> GKPRPYSPRPTSH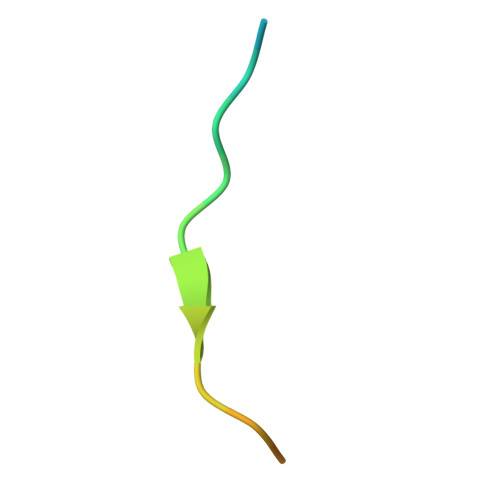PRPIRV>[4x]ILEAAVTQSPRNKVAVTGEKVTLSCQQTNNHNNMYWYRQDTGHGLRLIHYSYGVGNTEKGDIPDGYEASRPSQEQFSLILVSATPSQSSVYFCASGVGGTLYFGAGTRLSVL;>ESQPDPMPDDLHKSSEFTGTMGNMKYLYDDHYVSATKVKSVDKFLAHDLIYNISDKKLKNYDKVKTELLNEDLAKKYKDEVVDVYGSNYYVNCYFSSKDNVWWHGKTCMYGGITKHEGNH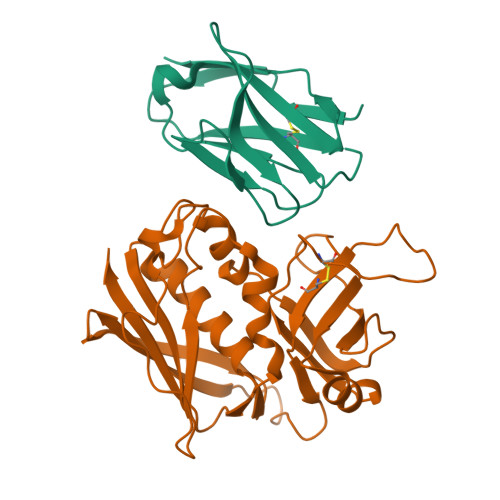FDNGNLQNVLVRVYENKRNTISFEVQTDKKSVTAQELDIKARNFLINKKNLYEFNSSPYETGYIKFIENNGNTFWYDMMPAPGDKFDQSKYLMMYNDNKTVDSKSVKIEVHLTTKNG[4x]>[2x]EEDKAYWNKDAQDALDKQLGIKLREKQAKNVIFFLGDGMSLSTVTAARIYKGGL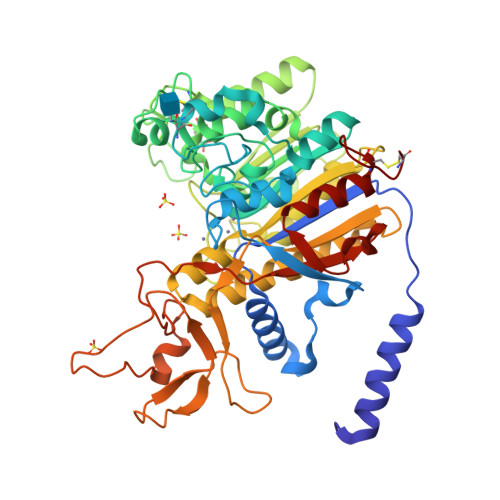TGKFEREKISWEEFDFAALSKTYNTDKQVTDSAASATAYLTGVKTNQGVIGLDANTVRTNCSYQLDESLFTYSIAHWFQEAGRSTGVVTSTRVTHATPAGTYAHVADRDWENDSDVVHDREDPEICDDIAEQLVFREPGKNFKVIMGGGRRGFFPEEALDIEDGIPGEREDGKHLITDWLDDKASQGATASYVWNRDDLLAVDIANTDYLMGLFSYTHLDTVLTRDAEMDPTLPEMTKVAIEMLTKDENGFFLLVEGGRIDHMHHANQIRQSLAETLDMEEAVSMALSMTDPEETIILVTADHGHTLTITGYADRNTDILDFAGISDLDDRRYTILDYGSGPGYHITEDGKRYEPTEEDLKDINFRYASAAPKHSATHDGTDVGIWVNGPFAHLFTGVYEENYIPHALAYAACVGTGRTFCD> MANLDRRKMMMLSGLGVMAAALPAPHAQALPTKPQTPPVPVPSAPQAAVNYVFADEFDGPAGSSPNTSKWTIAKARETIKDPTYWEQPGRIGQYRDDRKNAFLDGKGNLVIRATKEGDTYYGAKLASVWEGGAGHTWEARIKFNCLTAGAWPAFWLGTLGEGELDIVEWYGNGKWPSATTVHAKSNGGEWETHNIAVDTA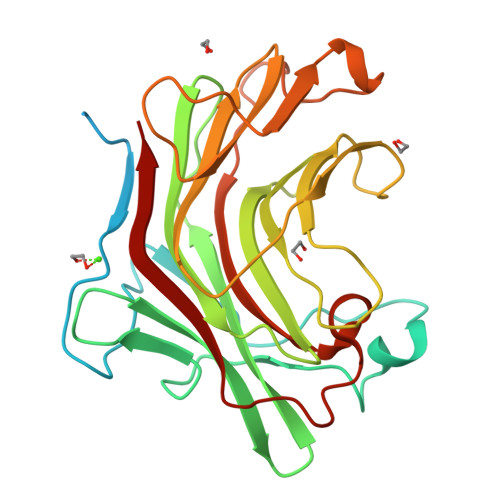WHTWRTQWDANGARFWQDYTEGAKPYFEVSASQLPDWPFNQPGYTMFVVLNLAVAGSGGEDPSGGTYPADMLVDYVRVW>MSRFIRASQRRTLLATLIAATLAQPLLAAESLDSKPASAITAAKNAEVLKNLPFADREEFEAAKRGLIAPFSGQIKNAEGQVVWDMGAYQFLNDKDAADTVNPSLWRQAQLNNIAGLFEVMPKLYQVRGLDPANMTIIEGDSGLVLIDTLTTAETARAALDLYFQHRPKKPIVAVVYSHSHIDHFGGARGIIDEADVKAGKVKVFAPSGFMEHAVSENILAGTAMARRGQYQSGVMVPRGAQAQVDSGLFKTTATNATNTLVAPNVLIEKPYERHTVDGVELEFQLTLGSEAPSDMNIYLPQFKVLNTADNAPPAMHNLLTPRGAEVRDAKAWAGYIDASLEKYGDRTDVLIQQHNWPVWGGDKVRTYLADQRDMYAFLNNRALNLMNKGLTLHEIAAEVSKLPGELDRKWYLRSYYGALSTNLRA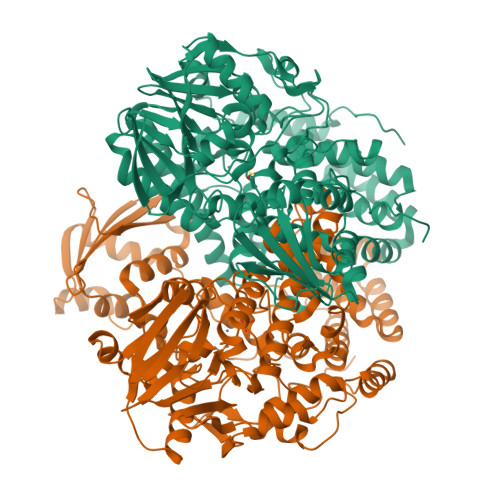VYQRYLGFYDGNPANLDPFPPVEAGKRYVEAMGGADAVLKQMRAAIDKGDYRWAVQLGNHLVFADPANKDARALQADAMEQLGYQTENALWRNMYMTGAMELRHGVPTYDSRGKSEMGRALTPDMFFDLLAIRLDTDKAVGHDMTLNWVFEDLKQDIALTLRNGVLTQRVGSLNPKADVTVKLTKPTLDQIAARKLDLPTAIKQGTVKLDGDGKKLGEFFGLLDSFSPKFNIVELEHHHHHH[6x]>SNAMEAFNSWLEGQNLKEQVKNPNIEVGDYSYYSGFYHSKTFEEQAVRYLLGDAPTQEVWESGQFGEVDKLRIGKFCSIASGATFMMAGNQGHRADWISTFPFSKKEFGEGVKDGFQRAGDTIVGNDVWIGSEAMIMPGVHIGDGAIIGARAVITKNVAPYSVVVGNNVVVKKRFDENLIQTLLVIKWWDWPLQHIKNTMEI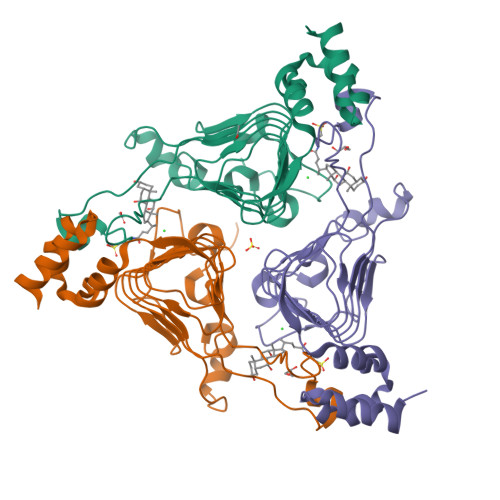LCSGHIEELEQYFIKNVGS[12x]2-METHYL-5-METHYLENE-5H-PYRIMIDIN-4-YLIDENEAMINE | C6 H7 N3 | 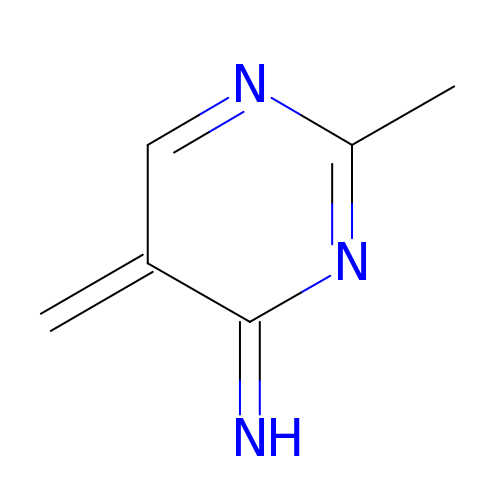AXFPKNUSOMMYRV-UHFFFAOYSA-N>[2x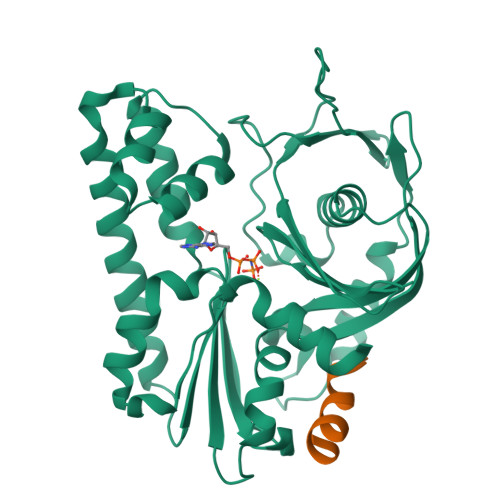]MLVFIDDGSTNIKLQWQESDGTIKQHISPNSFKREWAVSFGDKKVFNYTLNGEQYSFDPISPDAVVTTNIAWQYSDVNVVAVHHALLTSGLPVSEVDIVCTLPLTEYYDRNNQPNTENIERKKANFRKKITLNGGDTFTIKDVKVMPESIPAGYEVLQELDEADSLLIIDLGGTTLDISQVMGKLSGISKIYGDSSLGVSLVTSAVKDALSLARTKGSSYLADDIIIHRKDNNYLKQRINDENKISIVTEAMNEALRKLEQRVLNTLNEFSGYTHVMVIGGGAELICDAVKKHTQIRDERFFKTNNSQYDLVNGMYLIGN;>[2x]EQKSDEETKKNAMKLIN>MANGVIPPPGGASPLPQVRVPLEEPPLSPDVEEEDDDLGKTLAVSRFGDLISKPPAWDPEKPSRSYSERDFEFHRHTSHHTHHPLSARLPPPHKLRRLPPTSARHTRRKRKKEKTSAPPSEGTPPIQEEGGAGVDEEEEEEEEEEGESEAEPVEPPHSGTPQKAKFSIGSDEDDSPGLPGRAAVTKPLPSVGPHTDKSPQHSSSSPSPRARASRLAGEKSRPWSPSASYDLRERLCPGSALGNPGGPEQQVPTDEAEAQMLGSADLDDMKSHRLEDNPGVRRHLVKKPSRTQGGRGSPSGLAPILRRKKKKKKLDRRPHEVFVELNELMLDRSQEPHWRETARWIKFEEDVEEETERWGKPHVASLSFRSLLELRRTIAHGAALLDLEQTTLPGIAHLVVETMIVSDQIRPEDRASVLRTLLLKHSHPNDDKDSGFFPRNPSSSSMNSVLGNHHPTPSHGPDGAVPTMADDLGEPAPLWPHDPDAKEKPLHMPGGDGHRGKSLKLLEKIPEDAEATVVLVGCVPFLEQPAAAFVRLNEAVLLESVLEVPVPVRFLFVMLGPSHTSTDYHELGRSIATLMSDKLFHEAAYQADDRQDLLSAISEFLDGSIVIPPSEVEGRDLLRSVAAFQRELLRKRREREQTKVEMTTRGGYTAPGKELSLELGGSEATPEDDPLLRTGSVFGGLVRDVRRRYPHYPSDLRDALHSQCVAAVLFIYFAALSPAITFGGLLGEKTEGLMGVSELIVSTAVLGVLFSLLGAQPLLVVGFSGPLLVFEEAFFKFCRAQDLEYLTGRVWVGLWLVVFVLALVAAEGSFLVRYISPFTQEIFAFLISLIFIYETFYKLYKVFTEHPLLPFYPPEGALEGSLDAGLEPNGSALPPTEGPPSPRNQPNTALLSLILMLGTFFIAFFLRKFRNSRFLGGKARRIIGDFGIPISILVMVLVDYSITDTYTQKLTVPTGLSVTSPDKRSWFIPPLGSARPFPPWMMVAAAVPALLVLILIFMETQITALIVSQKARRLLKGSGFHLDLLLIGSLGGLCGLFGLPWLTAATVRSVTHVNALTVMRTAIAPGDKPQIQEVREQRVTGVLIASLVGLSIVMGAVLRRIPLAVLFGIFLYMGVTSLSGIQLSQRLLLILMPAKHHPEQPYVTKVKTWRMHLFTCIQLGCIALLWVVKSTAASLAFPFLLLLTVPLRHCLLPRLFQDRELQALDSEDAEPNFDEDGQDEYNELHMPV[2x]

Anion exchanger 3 (AE3) is pivotal in regulating intracellular pH across excitable tissues, yet its structural intricacies and functional dynamics remain underexplored compared to other anion exchangers. This study unveils the structural insights into human AE3, including the cryo-electron microscopy structures for AE3 transmembrane domains (TMD) and a chimera combining AE3 N-terminal domain (NTD) with AE2 TMD (hAE3NTD2TMD). Our analyzes reveal a substrate binding site, an NTD-TMD interlock mechanism, and a preference for an outward-facing conformation. Unlike AE2, which has more robust acid-loading capabilities, AE3’s structure, including a less stable inward-facing conformation due to missing key NTD-TMD interactions, contributes to its moderated pH-modulating activity and increased sensitivity to the inhibitor DIDS.

The structure of hAE3 in the presence of HCO3− and HCO3−/DIDS, and without HCO3− supplementation were determined with C2 symmetry, reaching overall resolutions of 2.7 Å, 2.7 Å, and 2.9 Å, respectively. In general, human AE3 adopts a homodimeric state, and each protomer is composed of a transmembrane domain (TMD) and an N-terminal cytoplasmic domain (NTD), the latter remaining unresolved in all three cryo-EM structures. In all three cryo-EM structures, hAE3 TMD consistently adopts an outward-facing conformation, demonstrating a high degree of structural conservation compared to human AE1 and AE2 in their respective outward-facing conformations. In TMDs, the cryo-EM density map was fragmentary for residues 860–883 in the extracellular loop at the dimeric interface and twenty-two residues of the C-terminal loop, and thus left unmodeled. In the AE3 TMD structures, the dimerization of hAE3 is primarily facilitated by hydrophobic interactions between the transmembrane helices TMH6 of the two protomers. Key residues oppositely arranged at the dimeric interface, including L894, I898, F905, and F909, form hydrophobic pairs that contribute significantly to the stability of the dimer. Notably, the contacts between the TMDs of hAE3 protomers are relatively sparse. Attempts to capture AE3 in its inward-facing state, similar to the methods used in resolving the full-length structure of AE227, including varying pHs and anions in cryo-EM sample preparation, did not yield alternative conformations of AE3. The inward-facing state of AE3 is suggested to be relatively unstable and transient, as inferred from the dominance of the outward-facing conformation in EM observations.Leucine aminopeptidase (LAP) is found in all kingdoms of life and catalyzes the metal-dependent hydrolysis of the N-terminal amino acid residue of peptide or amino acyl substrates. We report here the X-ray structures of three kinetoplastid acidic LAPs (LAP-As from Trypanosoma brucei, Trypanosoma cruzi, and Leishmania major) which were solved in the metal-free and unliganded forms, as well as in a number of ligand complexes, providing insight into ligand binding, metal ion requirements, and oligomeric state. LAPs of the M17 family of aminopeptidases are bilobal proteins with a highly conserved C-terminal domain harboring the aminopeptidase activity. They form homohexamers of approximately 330 kDa with the active sites facing a central cavity separated from the bulk solvent but accessible through solvent channels.

TcLAP-A crystallized only under citrate-containing conditions, resulting in crystals in space group R32 with one or both metal ions missing from the active site. TcLAP-A crystallized exclusively under citrate-containing conditions, which led to the absence of one or both Mn2+ ions from the active site and hence no electron density for the inhibitors. Apo TcLAP-A and the other LAP-A structures show completely ordered active sites independent of metal or ligand binding. In TcLAP-A, some loop regions in the N-terminal domain (between α2 and β2, β3 and β4, α5 and β5, and α6 and β6) and in the C-terminal domain (between β8 and β9 and between β10 and α11) show conformations slightly different from those in TbLAP-A. The corresponding residue numbers in TcLAP-A are K288, D293, D311, D370, and E372, and those in LmLAP-A are K299, D304, D322, D389, and E391. The analysis of TcLAP-A showed the presence of two well-separated peaks, one with a calculated molecular mass of ~320 kDa and the other with a mass of ~170 kDa, corresponding to the hexamer and trimer, respectively. At all of the concentrations analyzed, the hexamer was the most abundant species, while as the concentration was lowered, the proportion of trimers increased.

>MNRPPATDSGASEFVRSCVNFETNVEFTDVDAYKKTHTAGLASTFVVILGTHAQLREDALKELPFYCPAVAEAIQRVKKGETYAVLAEGVKNEANERFVRVLVGEVPSEASRTNCPARPDVVASLLSAALEEIKGPETKVDVFVRSTAALAIAVAAARSAKRNFTAKEGLATRGYCDNCVRLTVVFPTAPNPSPSELAVVATSTQLCQRLVDAPTNLLNTATFAEVAQSYAKELGCAVDVICGEELRERGYGGIYSVGKCAVEAPRLVTLSYKPKDETRKKVALVGKGIVYDSGGLSLKPTNFMTGMKRDMGGAAAVFCGFLTAVRLQMPIELSCTLCLAENAIGPDAYRNDDILTLKSGKTVEVNNTDAEGRLVLGDGVFHATHEISFKPDVLVDMATLTGAQGIATGHRHAGIFVNDEEEELSFLKAGRASGETCFPVLYCPEYHVTEFRSPVADMRNSVKQVNNASVSCAGQFVANHLSPDFKGKHIHVDMAFPAFENDKATGFGPALLTEYLRNLR[2x]>SMEATPCIKAISPSEGWTTGGATVIIIGDNFFDGLQVVFGTMLVWSELITPHAIRVQTPPRHIPGVVEVTLSYKSKQFCKGAPGRFVYTALNEPTIDYGFQRLQKVIPRHPGDPERLPKEVL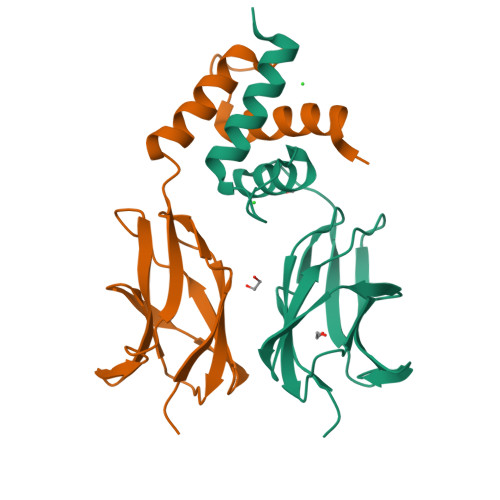LKRAADLVEALYGMPH[2x]>MTKKIHINAFEMNCVGHIAHGLWRHPENQRHRYTDLNYWTELAQLLEKGKFDALFLADVVGIYDVYRQSRDTAVREAVQIPVNDPLMLISAMAYVTKHLAFAVTFSTTYEHPYGHARRMSTLDHLTKGRIAWNVVTSHLPSADKNFGIKKILEHDERYDLADEYLEVCYKLWEGSWEDNAVIRDIENNIYTDPSKVHEINHSGKYFEVPGPHLCEPSPQRTPVIYQAGMSERGREFAAKHAECVFLGGKDVETLKFFVDDIRKRAKKYGRNPDHIKMFAGICVIVGKTHDEAMEK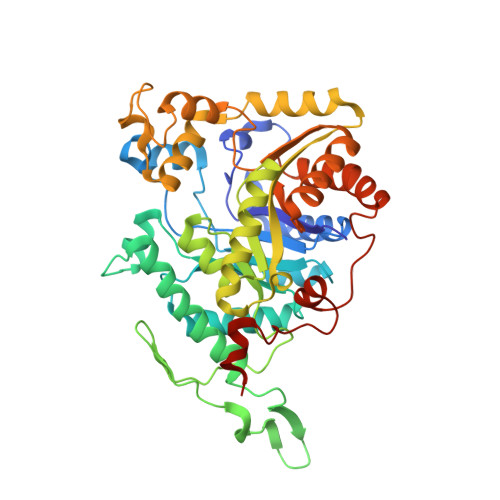LNSFQKYWSLEGHLAHYGGGTGYDLSKYSSNDYIGSISVGEIINNMSKLDGKWFKLSVGTPKKVADEMQYLVEEAGIDGFNLVQYVSPGTFVDFIELVVPELQKRGLYRVDYEEGTYREKLFGKGNYRLPDDHIAARYRNISSNV[2x]> VHFHPFGNVNFYEMDWSLKGDLWAHDPVIAKEGSRWYVFHTGSGIQIKTSEDGVHWENMGWVFPSLPDWYKQYVPEKDEDHLWAPDICFYNGIYYLYYSVSTFGKNTSVIGLATNQTLDPRDPDYEWKDMGPVIHSTASDNYNAIAPNVVFDQEGQPWLSFGSFWSGIQLIQLDTETMK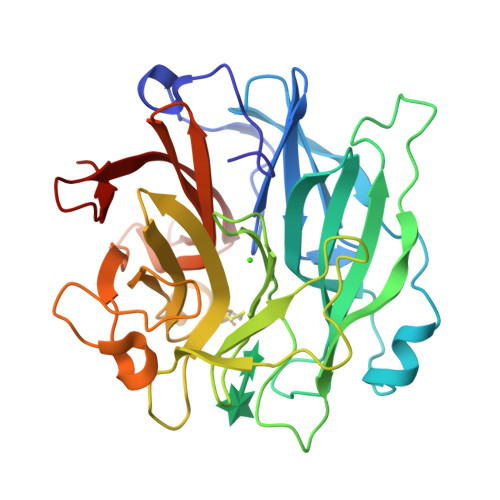PAAQAELLTIASRGEEPNAIEAPFIVCRNGYYYLFVSFDFCCRGIESTYKIAVGRSKDITGPYVDKNGVSMMQGGGTILDEGNDRWIGPGHCAVYFSGVSAILVNHAYDALKNGEPTLQIRPLYWDDEGWPYLSV> MYGLVNKAIQDMISKHHGEDTWEAIKQKAGLEDIDFFVGMEAYSDDVTYHLVGAASEVLGKPAEELLIAFGEYW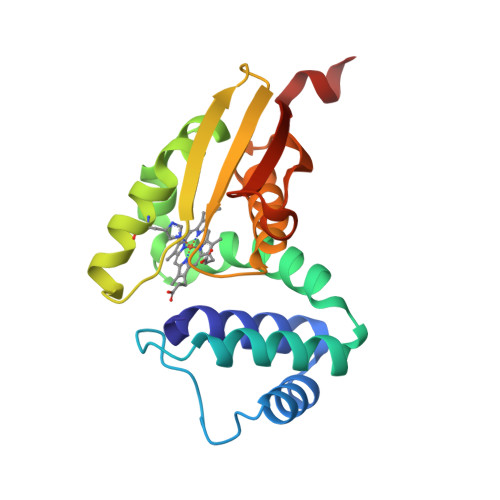VTYTSEEGYGELLASAGDSLPEFMENLDNLHARVGLSFPQLRPPAFECQHTSSKSMELHYQSTRCGLAPMVLGLLHGLGKRFQTKVEVTQTAFRETGEDHDIFSIKYEGAENLYFQ>[2x]TLRRRYTMVHQESLPNSTANSVDRQVGYFADNGVGNPLAIVQHPAGIHKNGITYVSYQGPKEDPYIASYNHQTGQWQGPFRAGISELGRRDGGKKFDNHGKPTMLIDDEGYIHIFYGGHGGQASNGKNPLGNTHHGANKHAVSKRPYDISQWEDLNNITPFGTYNQAIKMDNGDIYLFFRHGAHRSDWVYQKSVDNGRTFASPVSFLKHKRRTDIDAVDSWYAWAGKGQGDNIIVSYDYHVCWDGGA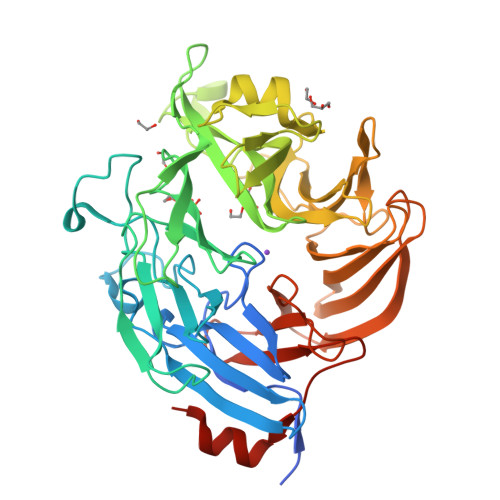GVNGRGHTTERHDVYFMSFNTKTGEWSNVEGEKLVLPVTREVADEKTMAMRTGELWTFNGSTHLDAQGQPHIAINAGIDKGAKTGGPKQTRHVRWNGNEWVGGDKVIPQYERVSRGDFMVTDPENIRYLTTYNQDNDAVLSWWQSHDGGEHFVEDKTVLRKDNASFAISAFIKDAIPDAQMLVAEKVSDEGIKMYLVGEEGAVTRSLVDLKTAMPTSKLEHHHHHH> GPGSKPFTLPILTIGELSNSRFPVPIDELYTSPNEGVIVQPQNGRSTLDGELLGTTQLVPSNICALRGRINAQVPDDHHQWNLQVTNTNGTPFDPTEDVPAPLGTPDFLANIYGVTSQRNPNNTCRAHDGVLATWSPKFTPKLGSVILGTWEESDL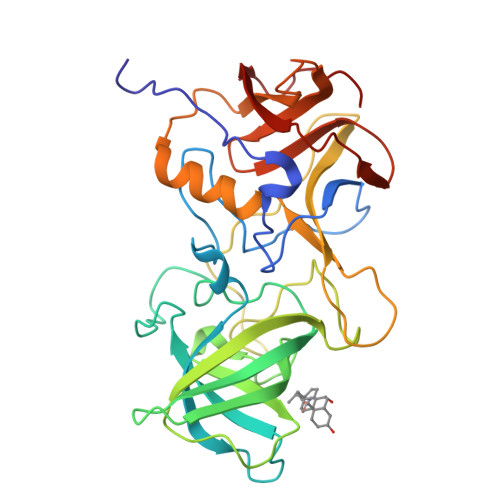DLNQPTRFTPVGLFNTDHFDQWALPSYSGRLTLNMNLAPSVSPLFPGEQLLFFRSHIPLKGGTSDGAIDCLLPQEWIQHFYQESAPSPTDVALIRYTNPDTGRVLFEAKLHRQGFITVANSGSRPIVVPPNGYFRFDSWVNQFYSLAPM>[2x]ANPLYQKHIISINDLSRDDLNLVLATAAKLKAN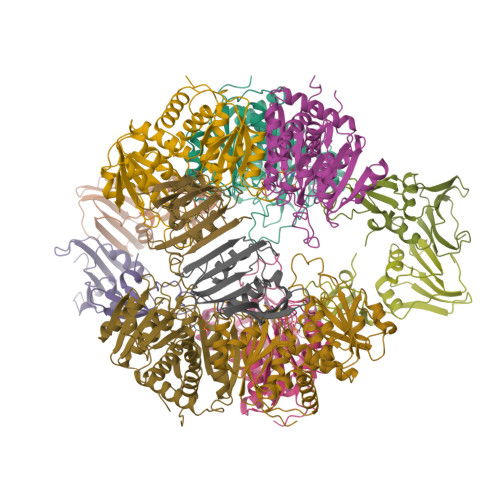PQPELLKHKVIASCFFEASTATRLSFQTSMHRLGASVVGFSDSANTSLGKKGETLADTISVISTYVDAIVMRHPQEGAARLATEFSGNVPVLNAGDGSNQHPTQTLLDLFTIQQTEGRLDNLHVAMVGDLKYGRTVHSLTQALAKFDGNRFYFIAPDALAMPEYILDMLDEKGIAWSLHSSIEEVMAEVDILYMTRVQKERLDPSEYANVKAQFVLRASDLHNAKANMKVLHPLPRVDEIATDVDKTPHAWYFQQAGNGIFARQALLALVLNRDLVL;>[2x]MTHDNKLGVEAIKRGTVIDHIPAQIGFKLLSLFKLTETDQRITIGLNLPSGEMGRKDLIKIENTFLSEDQVDQLALYAPQATVNRIDNYEVVGKSRPSLPERIDNVLVCPNSNCISHAEPVSSSFAVRKRANDIALKCKYCEKEFSHNVVLAN> MGEDLISQEDVVVTLSHQGYVKYQPLTDYEAQRRGGKGKSAARIKEEDFIDRLLVANTHDTILCFSSRGRLYWMKVYQLPEASRGARGRPIVNLLPLEANERITAILPVREYEEGVNVFMATASGTVKKTALTEFSRPRSAGIIAVNLNDGDEL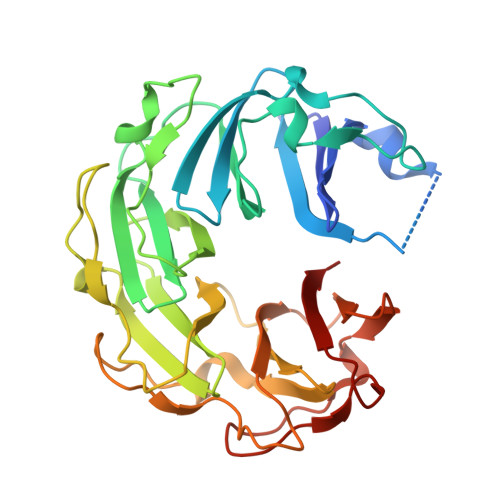IGVDLTSGSDEVMLFSAAGKVVRFKEDAVRAMGRTATGVRGIKLAGDDKVVSLIIPRGEGAILTVTQNGYGKRTAADEYPTKSRATQGVISIKVTERNGSVVGAVQVDDCDQIMMITDAGTLVRTRVSEISVVGRNTQGVILIRTAEDENVVGLQRVA> MVSTFPWLTVLWAVPVVGAAVVILLPAAQQVLAKWLALAVSVLTLAVTAVVAIGFDPAAAQYQFVESHRWIPSFGTGYILGVDGIALALVVLTAVLVPLLIIAGWNDASRQTGLAGRSVQAYLALTLAVEGMVLMSLVALDILLFYVFFEAMLIPMYFLIGGFGGENRSRAAVKFLLYNLFGGLIMLAAVIGLYVVTAGSDAFAAGTF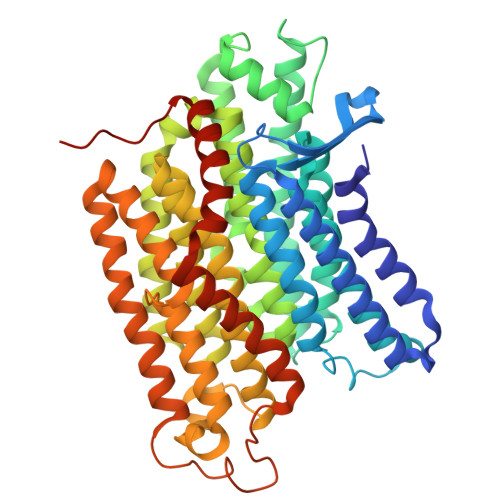DFREIVAAVSSGEFAVNPAIMNFLFLGFMFAFAVKAPLWPFHRWLPDAAVEATPASAVLMMAVMDKVGTFGMLRYCLQLFPDASTYFRPVVITLAAIGIVYGAVLAIGQTDVMRLIAYTSISHFGFIILGIFVMTSQGQSGSTLYMINHGISTAALFLIAGFLVSRRGSRLIDSYGGVQKVAPVLAGTFLVAGLATLSLPGLAPFISEFLVLIGTFTRYPVVAVFAATALVLSAVYILWTYQRMMTGPVRDGIGDGDRPVRDLVPRELVVVAPLLALLLVLGIYPKPALDVINPAVEHTLTTIGQTDPEPTVPPTIAEGAR>[4x]VESEPLYKLKAEFFKTLAH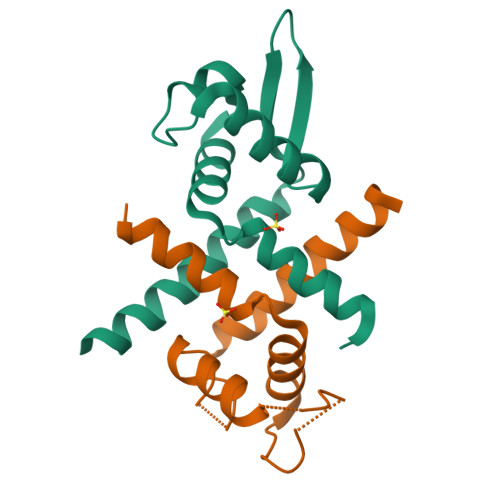PARIRILELLVERDRSVGELLSSDVGLESSNLSQQLGVLRRAGVVAARRDGNAMIYSIAAPDIAELLAVARKVLARVLSDRVAVLEDLRAGGSAT> GPLGSIPIEGRLQLKLGYDQNTLQLIVTLVCATGLSLRQSGAGRNPYAKVFLLPDRSHKSKRRTKTVGTTCEPRWGQTFVYSGLRRCDLNGRLLEVTL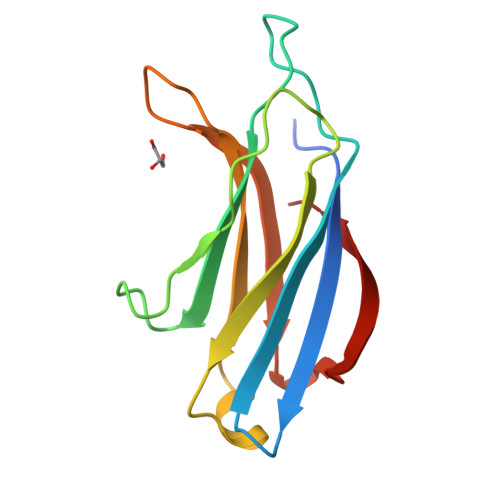WDYVRYGANDFIGEVVIDLAHHILDDEAEWYQLQ> MLTEGISIQSYDGHT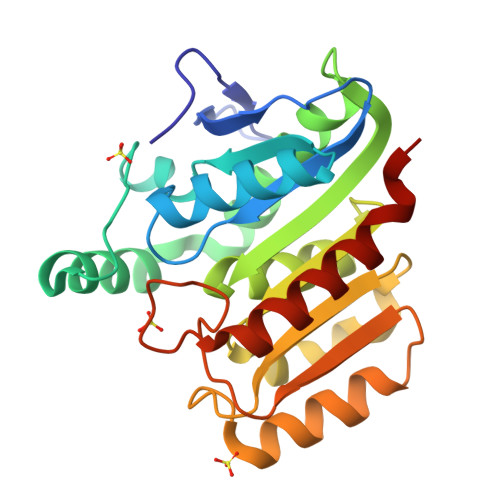FGALVGSPAKAPAPVIVIAQEIFGVNAFMRETVSWLVDQGYAAVCPDLYARQAPGTALDPQDERQREQAYKLWQAFDMEAGVGDLEAAIRYARHQPYSNGKVGLVGYSLGGALAFLVAAKGYVDRAVGYYGVGLEKQLNKVPEVKHPALFHMGGQDHFVPAPSRQLITEGFGANPLLQVHWYEEAGHSFARTSSSGYVASAAALANERTLDFLAPLQSKKP> MSMLKREDWYDLTRTTNWTPKYVTENELFPEEMSGARGISMEAWEKYDEPYKITYPEYVSIQREKDSGAYSIKAALERDGFVDRADPGWVSTMQLHFGAIALEEYAASTAEARMARFAKAPGNRNMATFGMMDENRHGQIQLYFPYANVKRSRKWDWAHKAIHTNEWAAIAARSFFDDMMMTRDSVAVSIMLTFAFETGFGNMQFLGLAADAAEAGDHTFASLISSIQTDESRHAQQGGPSLKILVENGKKDEAQQMVDVAIWRSWKLFSVLTGPIMDYYTPLESRNQSFKEFMLEWIVAQFERQLLDLGLDKPWYWDQFMQDLDETHHGMHLGVWYWRPTVWWDPAAGVSPEEREWLEEKYPGWNDTWGQCWDVITDNLVNGKPELTVPETLPTICNMCNLPIAHTPGNKWNVKDYQLEYEGRLYHFGSEADRWCFQIDPERYENHTNLVDRFLKGEIQPADLAGALMYMSLEPGVMGDDAHDYEWVKAYQKKTNAA;> MSEQQPEALKPLKTWSHLAGNRRRPSEYEVVSTNLHYFTDNPERPWELDSNLPMQTWYKKYCFDSPLKHDDWNAFRDPDQLVYRTYNLLQDGQESYVQGLFDQLNDRGHDQMLTREWVETLARFYTPARYLFHALQMGSVYIHQIAPASTITNCATYETADHLRWLTHTAYRTRELANCYPDVGFGKRERDVWENDPAWQGFRELIEKALIAWDWGEAFTAINLVTKPAVEEALLQQLGSLAQSEGDTLLGLLAQAQKRDAERHRRWSSALVKMALEKEGNREVLQKWV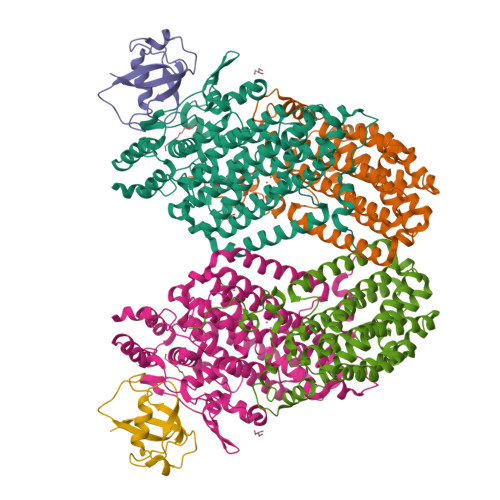AKWEPLADKAIEAYCSALPDGENAIVEAKSASRYVRQMMGL;> MATFPIMSNFERDFVIQLVPVDTEDTMDQVAEKCAYHSINRRVHPQPEKILRVRRHEDGTLFPRGMIVSDAGLRPTETLDIIFMDN(5S,6S)-6-amino-5-[(1-carboxyethenyl)oxy]cyclohexa-1,3-diene-1-carboxylic acid | C10 H11 N O5 | 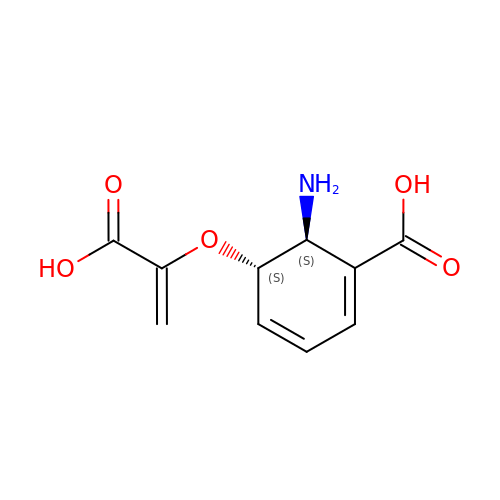OKLGKGPAZUNROU-YUMQZZPRSA-N~{N}-[[4-(diethylaminomethyl)phenyl]methyl]-4-pyrimidin-2-yl-piperazine-1-carboxamide 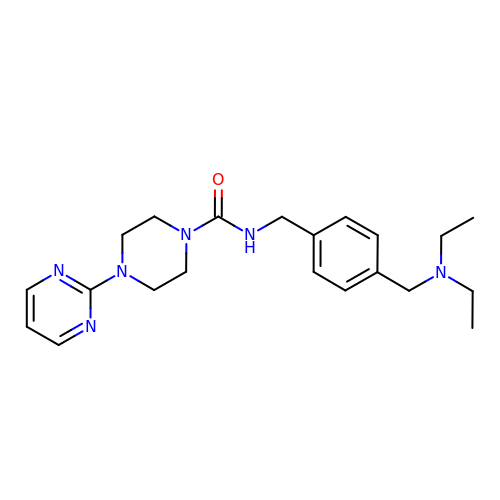| C21 H30 N6 O | BZUHDDVBSAICQG-UHFFFAOYSA-N> MAWRHLKKRAQDAVIILGGGGLLFASYLMATGDERFYAEHLMPTLQGLLDPESAHRLAVRFTSLGLLPRARFQDSDMLEVRVLGHKFRNPVGIAAGFDKHGEAVDGLYKMGFGFVEIGSVTPKPQEGNPRPRVFRLPEDQAVINRYGFNSHGLSVVEHRLRARQQKQAKLTEDGLPLGVNLGKNKTSVDAAEDYAEGVRVLGPLADYLVVNVSSPNTAGLRSLQGKAELRRLLTKVLQERDGLRRVHRPAVLVKIAPDLTSQDKEDIASVVKELGIDGLIVTNTTVSRPAGLQGALRSETGGLSGKPLRDLSTQTIREMY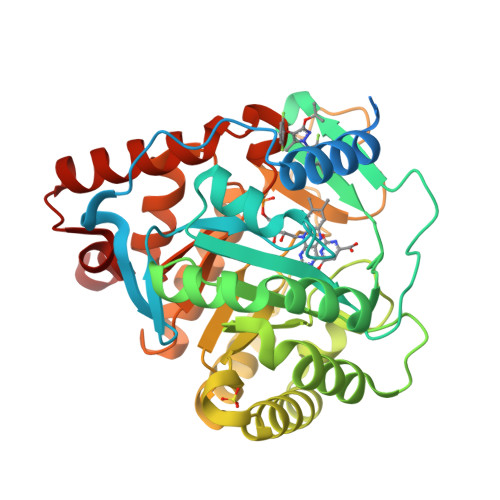ALTQGRVPIIGVGGVSSGQDALEKIRAGASLVQLYTALTFWGPPVVGKVKRELEALLKEQGFGGVTDAIGADHRR L-histidinol | C6 H12 N3 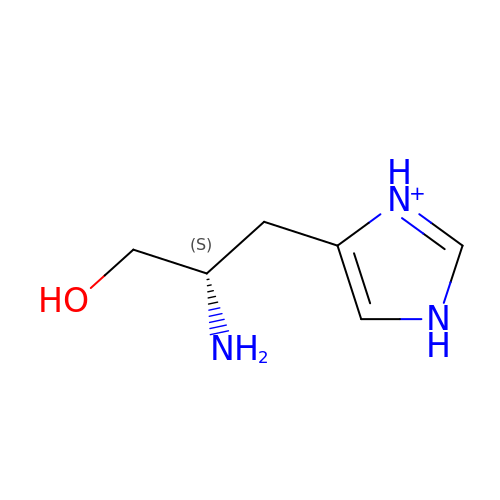O | ZQISRDCJNBUVMM-YFKPBYRVSA-O> MHHHHHHSYSYEACFWDPNDNGVNILLGHISQGIRSCDSMILFFKQRSELEKDYARRLGAITGKLDKDIGTNMDYGKLNETFNVVLSVEKARAQSHSKQSEILFRQIYTDTKAFAANLQARYTTLSGKIERLRMDKFNKKKGCEVLQKKLQDAQIRFRDLQLNENN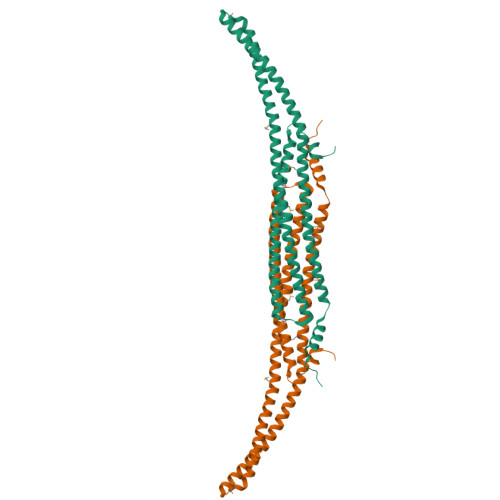MIGAKRVEHNKRELLKWESNSQEYKVQLDVLKQEYKASQKFWIHEWAQLSCELQEMENARISFLQSKLQQFATSSMETYILEQTKMDMLTNHLNSFTAADEISTFSKENGTGRLKHKTSKGDMNSSANWAQMSSISTTSK> SASRDDWRAARSMHEFSAKDIDGHMV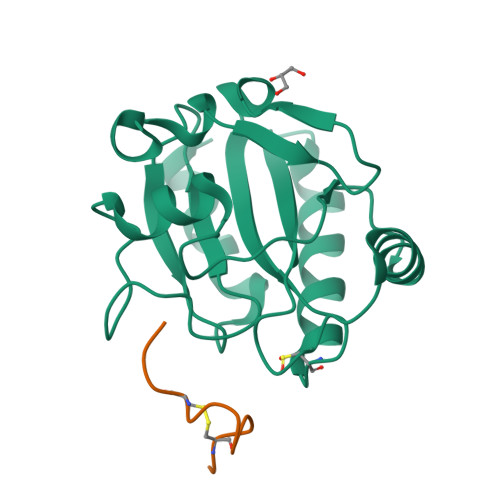NLDKYRGFVSIVTNVASQCGKTEVNYTQLVDLHARYAERGLRILAFPSNQFGKQEPGSNEEIKEFAAGYNVKFDMFSKIEVNGDDAHPLWKWMKIQPKGKGILGNAIKWNFTKFLIDKNGVVVKRYGPMEEPLVIEKDLPHYF;> VPCPYLPLWNCAGK> MDLIQAAYFVVAILFIVGLKRMAHPTTAKSGIVWAGWGMVLAVLATFFWPGMGNFALILLALLLGSVVAWWAAVRVAMTDMPQMVAIYNGMGGGAAATIAAVELLKGAFENTGLMALAILGGLIGSVAFTGSLIAFAKLQGIMKSRPILFPGQKAVNALVLALTVVIGLSLLWNDATASIVLFFLLALLFGVLMTLPIGGGDMPVAISFYNAFTGMAVGFEGFAVGNPALMVAGTLVGAAGT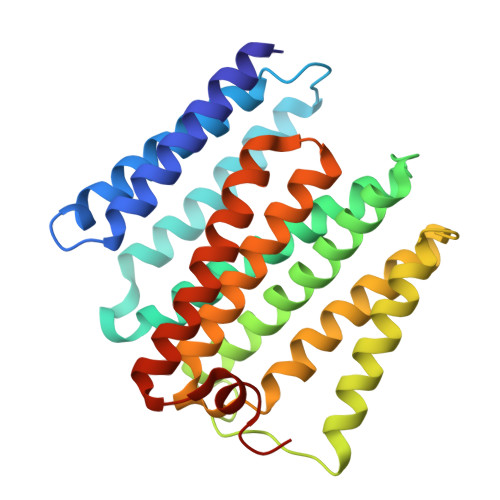LLTVLMARAMNRSVWISVLVGGHHHHHH>MFLFFFCDLFWLRLLLCMYYCVWSRLCFIVYFNCLMLIFDFLLFCLFDLYLFVGLCLFLLLWFMLFNLYSLILYYCITYLNLYLLFCIVFLLYIAFLFLFCFLCDFFLFNNLLVGDSFMDVFFIRFLLCFLECFSLLCRCLSTFLRLFCNLLSSHFLLLMFFDFFYFIFVFFFYGVFCYWFILFIFVFCFCLLFYVFLYLLDLFAAILQLFIFCNMILQLIMDFLLFLLFV[2x];>[6x]MRRFGSKFASGLASRCALACPLASAATAPAGASTTSSTSSAQKSFFKTTEMIGYVHSIDGTIATLIPAPGNPGVAYNTIIQIQVSPTTFAAGLVFNLEKDGRIGIILMDNITEVQSGQKVMATGQLLHIPVGAGVLGKVVNPLGHEVPVGLVTRSRRLLDSTLGKVDTGAPNIVSRSPVNYNLLTGFKAVDTMIPIGRGQRELIVGDRQTGKTSIAVSTIINQVRINQQILSKNAVISIYVSIGQRCSNVARIHRLLQSYGALRYTTVMAATAAEPAGLQYLAPYAGVTMGEYFMNRGRHCLCVYDDLSKQAVAYRQISLLLRRPPGREAYPGDVFYLHSRLLERAAMLSPGKGGGSVTALPIVETLSNDVTAYIVTNVISITDGQIYLDTKLFTGGQRPAVNIGLSVSRVGSSAQNAAMKGVAGKLKGILAEYRKLAADSVGGQQVQTIPMIRGARFVALFNQKQPSYFMNAIVSLYACLNGYLDDVKVQYVKFYEYLLVHRDLGIMYGTAKNKFFYMYVQELNYLIRFFTLNSPILHGELEEMLKQHTHLFLQHYQSKMNAIKSEKDVKALKNLLYSCKRAV;>[2x]MLRRLGANVSNMARPMNKYAVTVSPRRHLEPMSTWYLASWAMVWYYAFFFWMPMVWTDIMVPSFVYNKLPVIHFLQEKRAEQKLRRVLDETYTEWTEELDQAHVTDAITRSLNI;>MRRVSSPNITIQSVRWISGVSPLLYFPPTTTSTTNREDQINKNTNIAIQMIKRYKGEVPPHYTRKSSATIEQVEKEIDALLGGAEKLRKTSTDDQPMDKLTLMERCLRHALWSYHKEEGRYDFDQIGRWVVYTPEDEVKLAQLKREVEAKEKLAALRKRREEEGLPGGPVPRINWPQEYSSFIDREPVVAKRIRYDTLASTTLERDEKQIESTLQQYRRASQDKRLDDLVDLLERFKPVLAREAIMQRLTIKHLEGQLGVWRYMDWCPEVRDRAELEVDITGWQWWSPLEERRLLPVRLRSVNEVREIMSKTQAKKSAEAAERNPIVTQTSTGDNARDRLLKEVLALQARINQRDEVEPSQTEQKKKAHH[2x];>[6x]MLTRFRSAVLRGAVSITGARAASTAPVADHKGRVGHVSQVIGAVVDVHFADGVPPVLTALDVVDKLGRDEPLTLEIVQHLDAHTGRCIAMQTTDLLKLKAKVVSTGGNISVPVGRETLGRIFNVLGDAIDQRGPVGEKLRMPIHAVAPKLADQAAEDAVLTTGIKVIDLILPYCKGGKIGLFGGAGVGKTVIIMELINNVAKGHGGFSVFAGVGERTREGTDLYLEMMQSKVIDLKGESKCVLVYGQMNEPPGARARVAQSALTMAEYFRDVEGQDVLLFIDNIFRFTQANSEVSALLGRIPAAVGYQPTLAEDLGQLQERITSTTKGSITSVQAVYVPADDITDPAPATTFSHLDATTVLDRAVAESGIYPAVNPLECASRIMDPDVISVDHYNVAQDVVQMLTKYRELQDIIAVLGIDELSEEDKLIVDRARKLVKFLSQPFQVAEVFTGMTGHYVQLDDTIDSFSGLLMGTYDQVPEMAFYMVGGINSVLEKAKKMAEEAAELEKMRRARVAQASS;>MQGSWSVLKKNCSNFFPGLLAFAQQTQEAYGIWLRIYNRQQKYGPTDFVEQSETFSPDYHKRFHSQDKNMWVDKELCTEVSQKEVARLMTYKLDMWRMAHCAGALLATGGYAIPFGLFWLANDTWVPSSFNLTGEELRAWREAQDLYRYRSAPSYLTDTKWHFDFHAYPWNETQERAWDDLFEKNDVRRDPKVVRPAAEMYDGFIKFELIRRKSLRHLCRSMNIPTFPMLARLCNGTRVRDYWNLAWCEDYMVITQRLHESMTDEELYDYAWRRYLAPYDKNLNREQLMERVEDYFEFLGPDFVAHGKAPNLVILTNYVLGYYNDPAYLEGDISELDKNDYDHLASWGKDAFLRRLEFENGPLRDQVEAHTQRLLAERAAIAKGDNAAAVEGRHTA[2x];>[2x]MVLFSTYRSSRLVSKEFLHGPVMRFRALGEYYFQRAWNGTLNWALPGEYRLYAV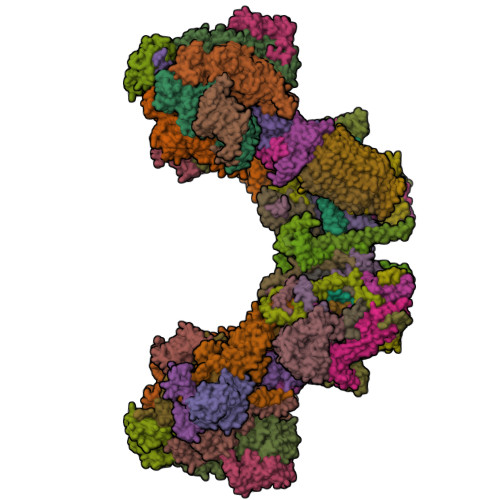MIPFIYFYHRWHNDHTLDRDHVEKAMIMRWGGTLEDVRKLSAKDQLRVRCFTDIEKLYSAYGPKDTYLQPPGDTLPGKDFYRKAGGAQAHH;>[2x]MSKQLTFISAGATAAVLQSASAIVSKVAGGRVQTKTAKEAGRHAVVVGPETPIGVHTAVTEVPKSAQDPLFSGVSTVVVRAVLPRAAPDSVQLRDALDVYASAGIDTKEEVRSATEAFKKSAEVAVGKAKAKGVKRIVLVVKQASKHNCINELFKKISTETIESAGLTTEVVGTAAVANQLIVNPESLGVVLLNDVAATEQIELAFAGVVGGVSRVYHTVEGGKISAGHSFKSVALAVAQELRELGLSSEADKVEAAASKNPRAVVSAL;>MSGKLRLYKEKLEGYNRFYSIVKTIKMVTLAKYRAAQGRIRTRDFSLRYTELAFSKPQASRDAVVAAKNALVYIPITTNRGSCGALNSNIVRCIDSVVSSKMVLMPVGKRGIDSFSKLYPDEFRYGIINDMKESMHFGYATFVIENAYEVSKDADRYQVIFNRFVSAGVQRNAVYNIPSYEKWKEDLADAASSDNQKNRYLFANALQNEEEQLIRDFFDFHAALAVLNAVGENELSEQAARLVAVEGQLTNISSLQQRTSSLYNKTRQFGITAALIEILSAMSSLEGNAMKGVRRNKFWEGAVTK[2x];>[2x]MRRTFISFSAASAAAAAPVTSTKMQTLHKLLTGEVSFKNKAPVKDCNIVHQFGENWATELSAYAKTLPAEQQKIIVRQIARVKLTRYTVAELAAYCGDGPALLDETARAANIEQGVAFVKAKGVEAFEKYVAEESTNANWKPEEAKKFIEDVKAKAK;>[2x]MFRTFGRRLVSCTLPLLQSAPHDLPEGFEFMEHKVVNKDIHAPHENLETLRLTLTRQDEFLLREEPVKCVTVTGTNGEYGIYPGHAYKIVQLNPSPLTVEYTDGTTKKYFVSGGFAHINNEGSCDVNTVECTLLDDLDLAIAEKELAAQQAALGSAKDDKAKSVVEIRISVIEAVIAALKHH;>MVYTRWKCDRLPVFQLKLFTQEYPMHAAVGIFTIIFLWKHMSHCSEETERKYGWWAGYPYWRDPIARRNETKYKQMIINNDVDITHPKWTGCSVEQLEELSRVV[2x];>MIRRSCALLSSSWRDHGISYLKYLNVCTETLHSTVKESRRAKYERWSKPCYTAQRPDGAGGQETIDKVPIHTKDY[2x];>[2x]MTKYELKMQYFDEWMIRWRKFQTESDWEIEKGRQWWRRFNMAVSGALFCGLVLYTSGTATLKRQYGLPHFFDIGVDGQAKETMLKTLTSRWRYTPQGYGRVLITGVPTYILFVTLEHYRERRRMQQYLQQNTVFGEQMRRLLSTGKIEEYLPVNIKATLPASQQAIYNY;>[6x]MMRRVYSPVFCSVAAARFAATSAAKKYDLFGYEVDTNTAPWIEKIKKCKYYDEAGEVLVNMNVSNCPPDIATYNATLQCIYQSPSKQSTPVDNESKFCAMMDLLEEMQHRNRLKPNEESWTWVMKECVKSGQFRLGYCIQQVMETECKGCPADLVKANEANAQKAKTEGKEHPGHLSQQAGLFDVKVE;>[2x]MLRRSSAALIRRTPVRHSGGELFVRPKLEEIPPADQCRGFFGPLNDSLKFLRLLDIKWMMNRAVAMRREYLIATPTLFTFIWMFTWKGAVIYFWGDRAPPRRMDWNTEETGRLPLGFKPTPAPL;>[2x]MSAKAAPKTLHQVRNVAYFFAAWLGVQKGYIEKSANDRLWVEHQRKVRQQNVERQQALDSIKLMQQGVRATTPGQLEGVPAELQQLAEAFTK;>[2x]MSSTKCAVACKIMTPLCNAASKVQARSAKKLAALTDAGIQKTISEHNANGTDAAVSSTKRYLAEQRQLFHYRVVRFFDECHYIISGEYFAQYTKVNLIWDLRFLTKLVVLFLIGTVLGRQSIFPPIDPDSPLVEALVTKVNPNY;>[2x]MFRRLSSSARAVVAARFYTPPEGLKKLYASDFENSKYPLNIVPSDSVLFAKFLYKAAEEKGNFDNILSDFQKIAAAASKLPIFWERTAVVEKIPEFKQLSEPTFFTLVWMQNNGMLELIQEVAEVYETFVNAKQKKAVAKIFVAPGGEKNVEEARRVAEELHKGLKELADYTLVLKTVVDRTIVKGFAVELAGQYVNKAEGQQKQAGRADEVDYTNLPAPKPQKTVWDDNIETEVLRKYLDGLSQYDMEEAKYGV;>[2x]MLRKTPLFAMATTRKALVGNGPTFSTGGECMNTCDIQNAFPMNDRGVRSSSPFQEPNTAIYDSYLAWTYFQPMDVHIEKLPAPEAKYYQRHTKKPWDVSSTELTEIQSRKKYFQTLGYLVAFIYLYFLMPKEKSFSGLSGPDGHWIMLPKGRPELF;>MSSGFHFHDVSNDAIKGMPPSEALHKHLENAQLAHRICLAKALKAGEPPVEKCALTWGEVLIRYQAWSEYRPPFQDSVAQAKYKKYWSKKRQEEDDKNPFK[2x];>[20x]MMRRLALQSSIRRATPFATPLVASTKALNPMCSAITIREASTVAISVQGLHYVGTGLAAIALAGVGLGIGTIFGNLLVACARQPNLTKMLFNYAILGFALTEAIGLFALMLAFLMLFS;>[2x]MLRRLVPRVMMAPMGGATALCTSRGYNMLVFRDPKRRPQLSEEERAKVVVNQAEWPEEFKDFDPDDPYKNSPEIIKGMSSWNLFLWGVECAFIYQFYELVFPKSI;>[2x]MTENIEAVMSDFWSNPADHFRPNLKALTLYAERQHYVDRWLHVKERWLAPWYLPWWSPLFQLGTWYSQRSRNLFLVENHLSYRPYKFRRNDEDRNNPY;>MLLGGFVPRRFSQFNRDPCWMFFIFSVGFWLGEYPAMMIKYNARDLVYDPHRYVWSHHDDHH[2x]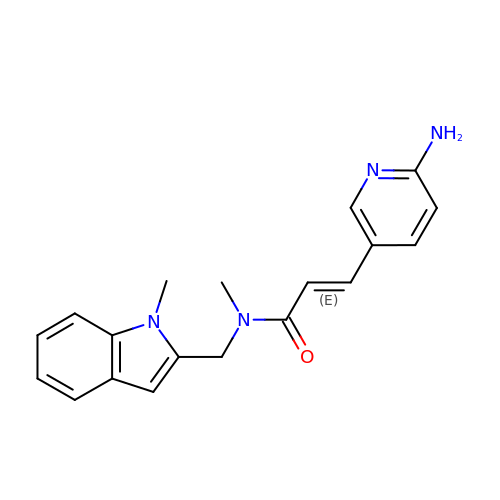3-(6-AMINOPYRIDIN-3-YL)-N-METHYL-N-[(1-METHYL-1H-INDOL-2-YL)METHYL]ACRYLAMIDE | C19 H20 N4 O | AKFPMLBVLWZSQX-CSKARUKUSA-N>ANKPMQPITSTANKIVWSDPTRLSTTFSASLLRQRVKVGIAELNNVSGQYVSVYKRPAPKPEGCADACVIMPNENQSIRTVISGSAENLATLKAEWETHKRNVDTLFASGNAGLGFLDPTAAIVSSDTT[178x];>[2x]MNMYKWVPESIRDSGEGQPSYSNNGDYAPSGPWVAAGIHTMPQSLRDSMRNSIMVTAQARRDVIGPEWGPDGRFTGYASVIGTPDPKPADIVNKFTVERRPVSNGNFQQRVKAGDIVVAPYTSDGKITVKLVAGQKDISSTPDYDYRIDSSLASSAGFVVAGERWYYTKRHFIIPRYFQNWRMRRRKYVTGWVMPTFYSPKEIFNRLKDSLVPDTGLVTQVWADNNTKRMDFLTAMAEIPQTLSSFLDALGYLGSLIKDFKRRRFFLNKAHQRIRNKLGVSFAERRSQIVSKYDRKIASARKPAIIVKLRQRKEKALKALDKMRVREEKKMIREFATQAASLWLSFRYEIMPLYYQSQDVLDVIANSTSEFMTSRDFVAKAINIGIPLEWNLDQENLVSQPRHNVMVKSKLSPENNIGKTLSVNPFTTAWELLTLSFVVDWFVNFGDVIAGFTGGYSDDSGATASWRFDDKKVFHLKNIPSAMVIVDINFYTRQVIDPRLCGGLAFSPKLNLFRYLDAMSLSWNRSRLKISRAT

Single-stranded RNA bacteriophages (ssRNA phages) are positive-sense RNA viruses that have shown specificity for gram-negative bacteria by exploiting host retractile pili, including T4P6. Acinetobacters have type IV pili (T4P), which are involved in twitching motility, surface adhesion, biofilm formation, and natural transformation in gram-negative bacteria. Our study delves into the interaction between Acinetobacter phage AP205 and type IV pili. Using cryo-electron microscopy, we solve structures of the AP205 virion with an asymmetric dimer of maturation proteins, the native Acinetobacter type IV pili bearing a distinct post-translational pilin cleavage, and the pili-bound AP205 showing its maturation proteins adapted to pilin modifications, allowing each phage to bind to one or two pili.

The smaller proportion of particles exhibiting a defined RNA organization, in contrast to MS2 (>90%)18 and Qβ (~30%), may be due to the more heterogeneous RNA conformations inside the capsid. Nonetheless, we achieved a 3.1Å-resolution asymmetric reconstruction of the mature AP205 virion, enabling us to construct a complete atomic model of both the capsid protein shell and the gRNA, which consists of 4,269 nucleotides. In our structure, 178 copies of the Coat self-assembled into a near-icosahedral shell (with the triangulation number, T=3), measuring approximately 290 Å in diameter. Surprisingly in contrast to MS2 and Qβ, which have a single Mat per virion, AP205 possesses a distinctive Mat-dimer, resembling the shape of the letter “F” at a pseudo two-fold axis of the capsid and increasing the length of the virion for an additional 70 Å. The two copies of Mat exhibit different conformations: One Mat (referred as outer Mat) extends further to elevate its apical domain away from the capsid shell while the other Mat (referred as inner Mat) is embedded deeper within the capsid and has a larger bending angle between the central and basal domains. These two Mat proteins intertwine to form hydrogen bonds and salt bridges at three sites. The third interaction is within a six-helix bundle between the two basal domains, connected by a salt bridge between Asp321 (α5 of the outer Mat) and Arg347 (α5 of the inner Mat). These interactions hold the two copies of AP205 Mat together, forming a dimer that nearly triples the volume and doubles the surface area compared to a single Mat in ssRNA coliphages. The 3’ region of the gRNA is proximal to the Mat-dimer on one side of the capsid, while the 5’ region resides on the opposite side. Notably, one RNA stem-loop originating from the 3’ end of the AP205 gRNA, which interacts with the Mat-dimer, is partially exposed outside the capsid shell. The AP205 gRNA is highly branched, presenting a total of 88 stem-loops, two of which provide specific interactions with the Mat-dimer via multiple π-stackings between aromatic amino acid sidechains and RNA bases.>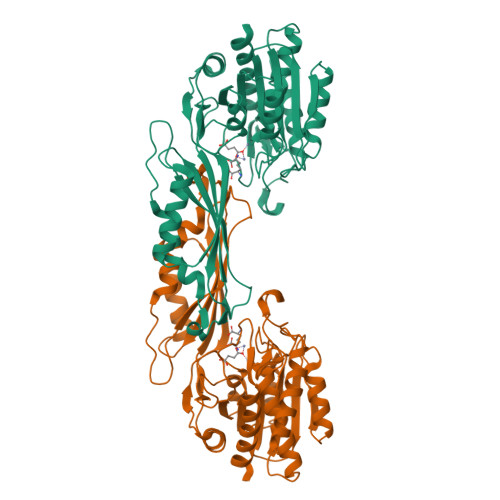 ASNAMKEKVVSLAQDLIRRPSISPNDEGCQQIIAERLEKLGFQIEWMPFNDTLNLWAKHGTSEPVIAFAGHTDVVPTGDENQWSSPPFSAEIIDGMLYGRGAADMKGSLAAMIVAAEEYVKANPNHKGTIALLITSDEEATAKDGTIHVVETLMARDEKITYCMVGEPSSAKNLGDVVKNGRRGSITGNLYIQGIQGHVAYPHLAENPIHKAALFLQELTTYQWDKGNEFFPPTSLQIANIHAGTGSNNVIPAELYIQFNLRYCTEVTDEIIKQKVAEMLEKHNLKYRIEWNLSGKPFLTKPGKLLDSITSAIEETIGITPKAETGGGTSDGRFIALMGAEVVEFGPLNSTIHKVNECVSVEDLGKCGEIYHKMLVNLLD>[2x]MSHHHHHHSMTQQQAKANGISINYEDRGPADGIPILLVNGYTSTMMSWPLELMDGLKARGFRVIRYDNRDVGRTEKFKGVPDIGEVVKALREGKTPETPYTLSDMAADGIGLMDALGIERAHVMGISMGGMIVQAMAINHPERLVSVTSIMSTTGNY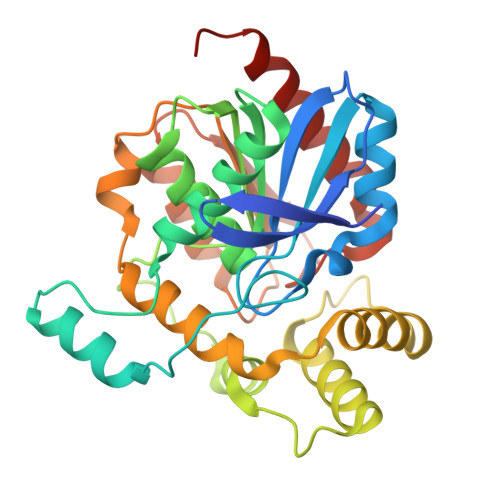DLPKASDEAMAALQQQPASHDREVVIRHRMKARRVYQSPAFPRSDEALYALCATEFDHMYYPEGASRQYAAIVGDGSRVERLKKVRVPFLVIHGKADPLVPVEGGIDTAKCVPGAKLELIEGMGHDLPVELCPRYVDLIAEHALAAGRKAAAE>[2x]MGSDKIHHHHHHENLYFQGMRTFRLVIACPDRVGIVAKVSNFLASHNGWITEASHHSDNLSGWFFMRHEIRADTLPFDLDGFREAFTPIAEEFSMDWRITDSAQKKRVVLMASRESHCLADLLHRWHSDELDCDIACVISNHQDLRSMVEWHDIPYYHVPVDPKDKEPAFAE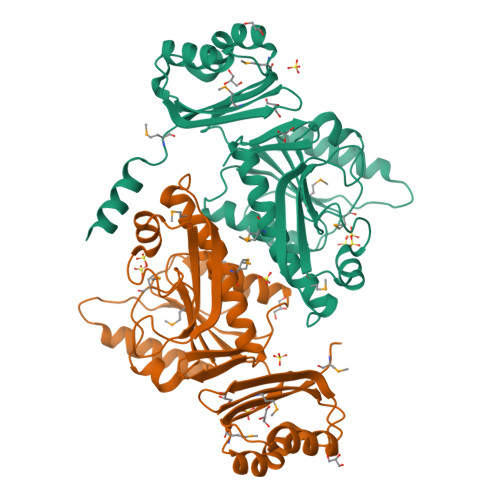VSRLVGHHQADVVVLARYMQILPPQLCREYAHQVINIHHSFLPSFVGAKPYHQASLRGVKLIGATCHYVTEELDAGPIIEQDVVRVSHRDSIENMVRFGRDVEKMVLARGLRAHLEDRVLVHDNKTVVFD> MGVTCVSQMPVAEGKSLQQTVELLTKKLEMLGAEKQGTFCVDCETYHTAASTLGSQGQAGKLMYVMHNSEYPLSCFALFENGPCLIADTNFDVLMVKLKGFFQSAKASKIETRGTRYQYCDFLVKVGTVTMGPSARGISVEVEYGPCVVASDCWSLLLEFLQSFLGSHAPGAPTVFGNRHDAVYGPADTMIQYMELFNKIRKQQQVPVAGI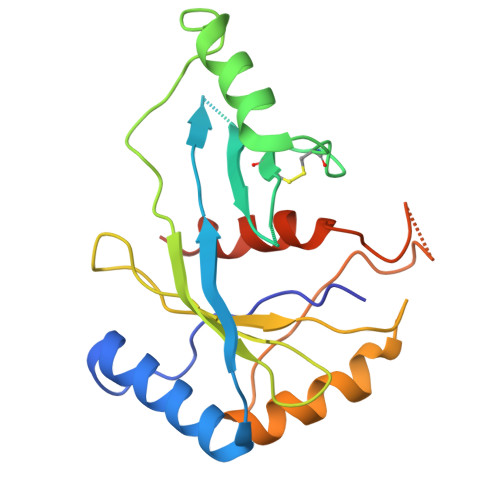R> KKPKNKDKDKKVPEPDNKKKKPKKEEEQKWKWWEEERYPEGIKWKFLEHKGPVFAPPYEPLPENVKFYYDGKVMKLSPKAEEVATFFAKMLDHEYTTKEIFRKNFFKDWRKEMTNEEKNIIT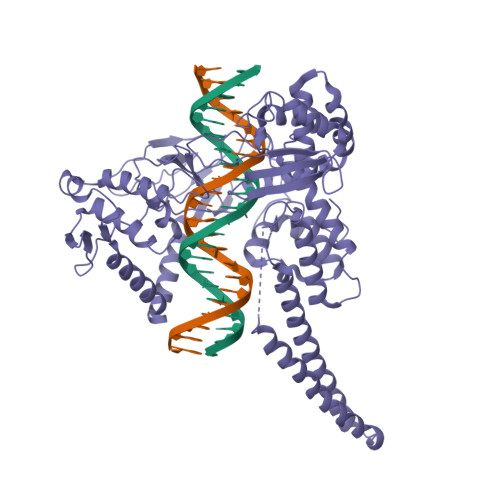NLSKCDFTQMSQYFKAQTEARKQMSKEEKLKIKEENEKLLKEYGFCIMDNHKERIANFKIEPPGLFRGRGNHPKMGMLKRRIMPEDIIINCSKDAKVPSPPPGHKWKEVRHDNKVTWLVSWTENIQGSIKYIMLNPSSRIKGEKDWQKYETARRLKKCVDKIRNQYREDWKSKEMKVRQRAVALYFIDKLALRAGNEKEEGETADTVGCCSLRVEHINLHPELDGQEYVVEFDFLGRDSIRYYNKVPVEKRVFKNLQLFMENKQPEDDLFDRLNTGILNKHLQDLMEGLTAKVFRTYNASITLQQQLKELTAPDENIPAKILSYNRANRAVAILCNHQRAPPKTFEKSMMNLQTKIDAKKEQLADARRDLKSAKADAKVMKDAKTKKVVESKKKAVQRLEEQLMKLEVQATDREENKQIALGTSKLNFLDPRITVAWCKKWGVPIEKIYNKTQREKFAWAIDMADEDYEF> MVEKEEAGGGISEEEAAQYDRQIRLWGLEAQKRLRASRVLLVGLKGLGAEIAKNLILAGVKGLTMLDHEQVTPEDPGAQFLIRTGSVGRNRAEASLERAQNLNPMVDVKVDTEDIEKKPESFFTQFDAVCLTCCSRDVIVKVDQICHKNSIKFFTGDVFGYHGYTFANLGEHEFVEEKTKVAKVSQGVEDGPDTKRAKLDSSETTMVKKKVVFCPVKEALEVDWSSEKAKAALKRTTSDYFLLQVLLKFRTDKGRDPSSDTYEEDSELLLQIRNDVLDSLGISPDLLPEDFVRYCFSEMAPVCAVVGGILAQEIVKALSQRDPPHNNFFFFDGMKGNGIVECLGPK;> SLMALSRGLPRELAEAVAGGRVLVVGAGGIGCELLKNLVLTGFSHIDLIDLDTIDVSNLNRQFLFQKKHVGRSKAQVAKESVLQFYPKANIVAYHDSIMNPDYNVEFFRQFILVMNALDNRAARNHVNRMCLAADVPLIESGTAGYLGQVTTIKKGVTECYECHPKPTQRTFPGCTIRNTPSEPIHCIVWAKYLFNQLFGEEDADQEVSPDRADPEAAWEPTEAEARARACNEDGDIKRISTKEWAKSTGYDPVKLFTKLFKDDIRYLLTMDKLWRKRKPPVPLDWAEVQSQGEETNASDQQNEPQLGLKDQQVLDVKSYARLFSKSIETLRVHLAEKGDGAELIWDKDDPSAMDFVTSAANLRMHIFSMNMKSRFDIKSMAGNIIPAIATTNAVIAGLIVLEGLKILSGKIDQCRTIFLNKQPNPRKKLLVPCALDPPNPNC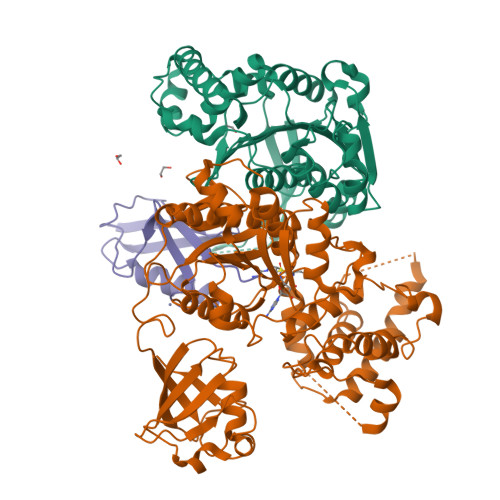YVCASKPEVTVRLNVHKVTVLTLQDKIVKEKFAMVAPDVQIEDGKGTILISSEEGETEANNHKKLSEFGIRNGSRLQADDFLQDYTLLINILHSEDLGKDVEFEVVGD;> MGSSHHHHHHSSGLVPRSHMSDQEAKPSTEDLGDKKEGEYIKLKVIGQDSSEIHFKVKMTTHLKKLKESYCQRQGVPMNSLRFLFEGQRIADNHTPKELGMEEEDVIEVYQEQCG>MKDLKGTKTAENLKQGFIGESMANRRYLYFAKRADEEGYPEIAGLLRSIAEGETAHAFGHLDFIRQGGLTDPATDKPIGTLEQMIESAIAGETYEWTQMYPGFAKVAREEGFPEVAEWFETLARAEKSHAEKFQNVLKQLKGGT[2x]

One such protein is sulerythrin (SulE), a ruberythrin-like protein isolated from the thermophilic archeon Sulfolobus tokodaii. SulE lacks the characteristic C-terminal, rubredoxin-like FeS4 domain of ruberythrins and contains a binuclear metal centre that coordinates iron and zinc when isolated from S. tokodaii. In contrast to other members of the ruberythrin family, a crystal structure of native SulE shows that it forms homodimers through domain swapping, with each monomer contributing two α-helices to give two four-helix bundles that each harbour a solvent-accessible, single dimetal site. The exact function of SulE is unknown, but it is presumed to be involved in reactions against oxidative stress.

In order to test the effect of the total absorbed dose on SpReAD analysis, data collection at higher flux values was repeated on the same crystal used at 5% beamline flux, choosing distinct, non-overlapping positions at least 50 µm apart. Data sets at 13.5 keV and nine energies over the rising Fe K edge were collected at 10% and 100% flux. Using RADDOSE-3D, the total average diffraction-weighted dose was calculated to be 0.26 MGy for 5% flux, 0.52 MGy for 10% flux and 2.70 MGy for 100% flux. Fe-2 and Fe-4 were therefore modelled in these distinct positions, with occupancies refining to 0.32 and 0.34, respectively, for position 2 close to His129 and 0.68 and 0.66, respectively, for position 1 equivalent to that occupied in the maps calculated from data at 5% and 10% flux. The SpReAD analysis was then repeated for the data collected at 10% and 100% beamline flux, refining the f′′ contribution for each of the two Fe-2 and Fe-4 positions observed at 100% flux separately. While there was no difference in the oxidation states of all iron ions between 5% and 10% flux, at 100% flux a clear difference was visible for Fe-2 and Fe-4 at position 2, where the edge position was coincident with Fe-1 and Fe-3, suggesting that iron ions at this position are reduced. Indeed, the total dose of 2.9 MGy taken up by the crystal at 100% beamline flux is close to doses that lead to photoreduction in other metalloproteins, such as insulin or heme-containing proteins. The study presented here shows that data-collection parameters that lead to a high total absorbed dose indeed result in a partial reduction of the metal in question, and that this is not only visible in the corresponding electron density but also in the SpReAD profiles.>SYYHHHHHHLESTSLYKKAGLMSTPLQGIKVLDFTGVQSGPSCTQMLAWFGADVIKIERPGVGDVTRHQLRDIPDIDALYFTMLNSNKRSIELNTKTAEGKEVMEKLIREADILVENFHPGAIDHMGFTWEHIQEINPRLIFGSIKGFDECSPYVNVKAYENVAQAAGGAASTTGFWDGPPLVSAAALGDSNTGMHLLIGLLAALLHREKTGRGQRVTMSMQDAVLNLCRVKLRDQQRLDKLGYLEEYPQYPNGTFGDAVPRGGNAGGGGQPGWILKCKGWETDPNAYIYFTIQEQNWENTCKAIGKPEWITDPAYSTAHARQPHIFDIFAEIEKYTVTIDKHEAVAYLTQFDIPCAPVLSMKEISLDPSLRQSGSVVEVEQPLRGKYLTV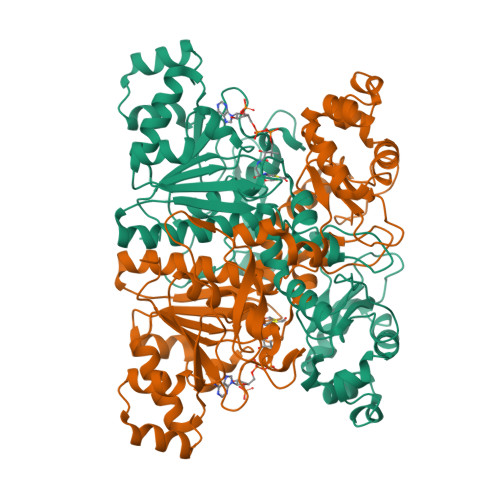GCPMKFSAFTPDIKAAPLLGEHTAAVLQELGYSDDEIAAMKQNHAI[2x]> MASGAARWLVLAPV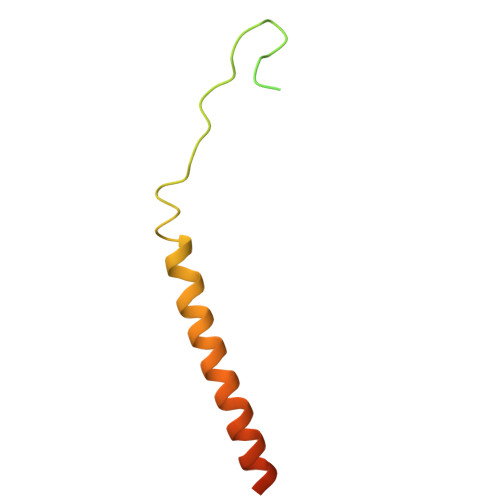RSGALRSGPSLRKDGDVSAAWSGSGRSLVPSRSVIVTRSGAILPKPVKMSFGLLRVFSIVIPFLYVGTLISKNFAALLEEHDIFVPEDDDDDD> MKKAVINGEQIRSISDLHQTLKKELALPEYYGENLAALWDALTGWVE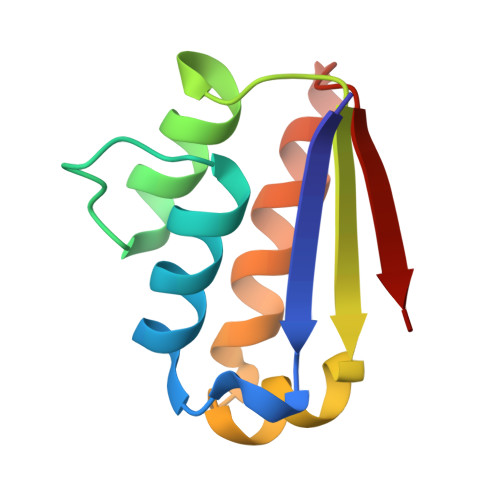YPLVLEWRQFEQSKQLTENGAESVLQVFREAKAEGADITIILS>[2x]AGSGLGRAYSGEGAIADDAGNVS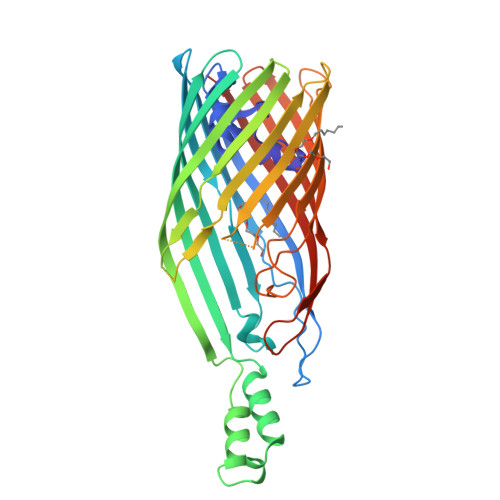RNPALITMFDRPTFSAGAVYIDPDVNISGTSPSGRSLKADNIAPTAWVPNMHFVAPINDQFGWGASITSNYGLATEFNDTYAGGSVGGTTDLETMNLNLSGAYRLNNAWSFGLGFNAVYARAKIERFAGDLGQLVAGQIMQSPAGQTQQGQALAATANGIDSNTKTAHLNGNQWGFGWNAGILYELDKNNRYALTYRSEVKIDFKGNYSSDLNRAFNNYGLPIPTATGGATQSGYLTLNLPEMWEVSGYNRVDPQWAIHYSLAYTSWSQFQQLKATSTSGDTLFQKHEGFKDAYRIALGTTYYYDDNWTFRTGIAFDDSPVPAQNRSISIPDQDRFWLSAGTTYAFNKDASVDVGVSYMHGQSVKINEGPYQFESEGKAWLFGTNFNYAFHHHHHH>AMALSGNEKHKENVAIENDGTPPRDKESLSPLTRFLNNELYGEKDARRKIGEITQTLLDHAVENGESQKVTLKGEAGRLTGYYHQGAASSEGETSATSGKVVLFLHGSGSSAEEQASEIRNHYQKQGIDMLAVNLRGYGESDGGPSEKGLYQDARTMFNYLVNDKGIDPSNIIIHGYSMGGPIAADLARYAAQNGQAVSGLLLDRPMPSMTKAITAHEVANPAGIVGAIAKAVNGQFSVEKNLKGLPKETPILLLTDNEGLGEEGEKLRAKLAIAGYNVTGEQTFYGHEASNRLMGQYAD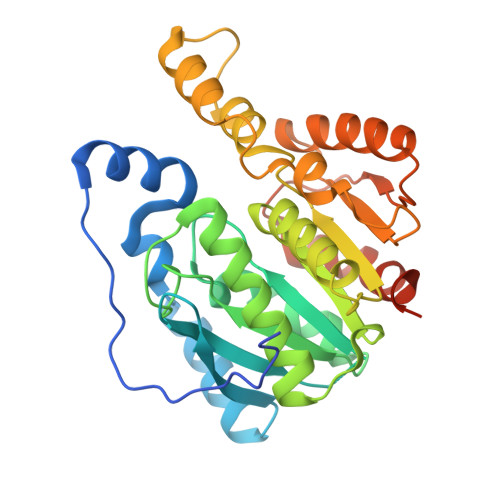QIVSGLFNAEQAAVEAGEVLKGL[2x]>SNAMDKIYIHDMEFYGYHGVFPEENKLGQRFKVDLTVELDLKRAGESDDLEHSVNYGELFELCRKVVEDRTYKLVESIAE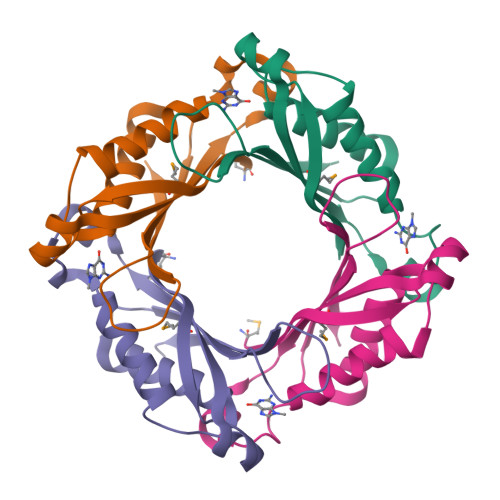NIATDILKQYESISRCTIKVIKPDPPIPGHYRAVAVEITRERP[8x]>MKNIFKIGLFALVTAFAMTSCDPQDGDDHSLGVKPQESQLSFTATPGSNPNVVTLKNTSSLKGLVVTWDLGNGVTAKGEEVVASYPFANTYTIAMTAYNTGGSTTITQTITIANNDESQIEPKAIILAGGLTGSKTWVFDRAHDGHFGVGPGAGNPDYNGTPSWWSCPAEGKAECALYENEFSFHLDGGYNMTWVNKGKIYTNGAGKDKLPGVATVPGAGDFDVEYIPKEAYTFTVDGDKLKLSDDAFFGHFAGTSTYT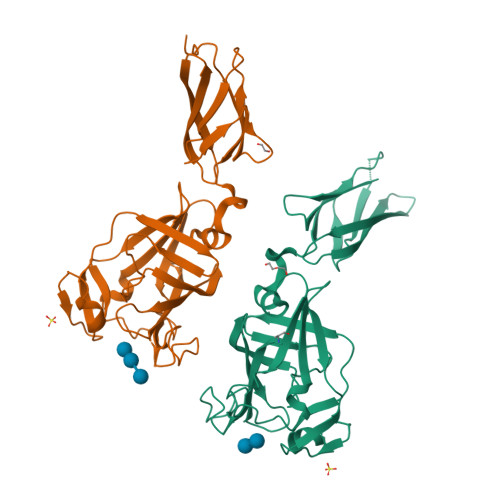IKTLNENELYLECSSAVESGNGWWYRFVPKK[2x]> NDETKALKELYGPVDPTFLHRFYSLKAAVHGWKMVVCDKVRSLKLSDNNCYLNAVIMTLDLLKDIKFVIPALQHAFMKHKGGDSTDFIALIMAYGNCTFGAPDDASRLLHTVLAKAELCCSARMVWREWCNVCGIKDVVLQGLKACCYVGVQTVEDLRARMTYVCQCGGERHRQLVEHTTPWLLLSGTP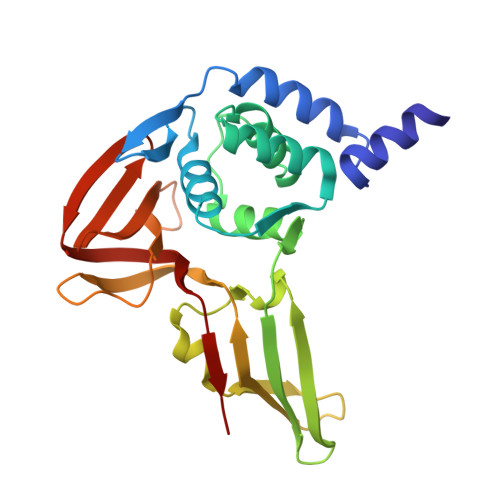NEKLVTTSTAPDFVAFNVFQGIETAVGHYVHARLKGGLILKFDSGTVSKTSDWKCKVTDVLFPGQKYSSD>[16x]XGELAALKQELAALKWELAALKEEL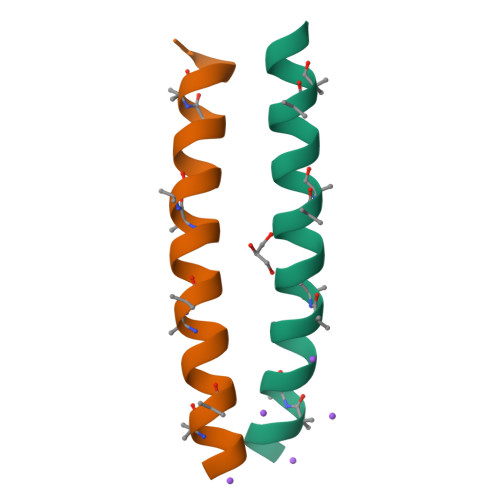AALKYGX> MSYSGERDNFAPHMALVPMVIEQTSRGERSFDIYSRLLKERVIFLTGQVEDHMANLIVAQMLFLEAENPEKDIYLYINSPGGVITAGMSIYDTMQFIKPDVSTICMGQAASMGAFLLTAGAKGKRFCLPN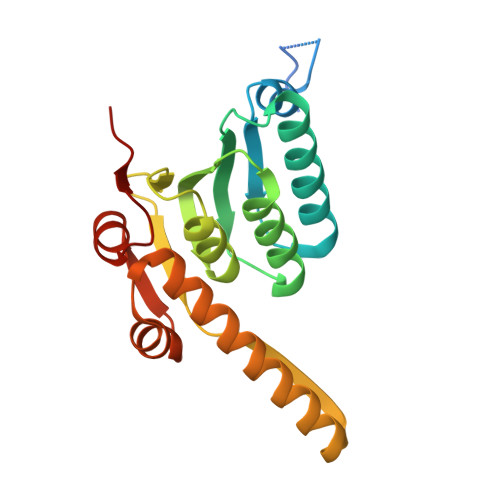SRVMIHQPLGGYQGQATDIEIHAREILKVKGRMNELMALHTGQSLEQIERDTERDRFLSAPEAVEYGLVDSILTHRN> MSDFDLIVVGSGLFGLTVAERAASQLGKKVLIVEKRSHLGGNAYSEAEPETGIEIHKYGAHLFHTSNKRVWDYVNQFTAFTGYQHRVFAMHNGTAYQFPMGLGLINQFFGRYYTPDEARELIKEQSAEIDSKDATNLEEKAISLIGRPLYEAFIRDYTAKQWQTDPKELPAGNITRLPVRYNFDNRYFNDTYEGLPVDGYAQWLSNMADHENIEVRLDTDWFEVREDLRAQNPEAPVVYTGPLDRYFDYSEGHLGWRTLDFETEVLNTGDFQGTPVMNYNDAEFPYTRIHEFRHFHPEREDRHPKDKTVI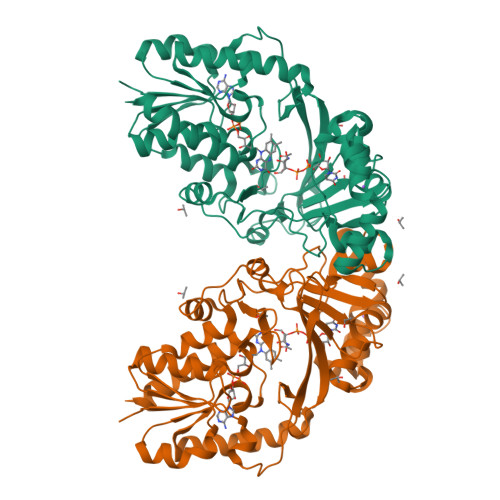MKEYSRFAEEGDEPYYPINTPSDREMLFKYRELADAETESGKVYFGGRLGTYQYLDMHMAIASALSMFDNKLVDALKHHHHHH> MHHHHHHGSKSVPTAEETRRLAQAM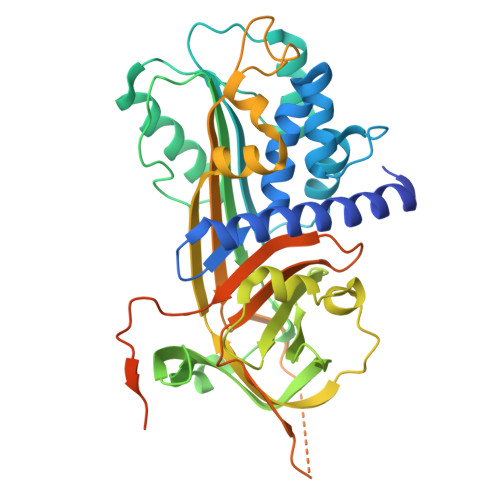MAFTTDLFSLVAQTSTSSNLVLSPLSVALALSHLALGAQNQTLHSLHRVLHMNTGSCLPHLLSHFYQNLGPGTIRLAARIYLQKGFPIKDDFLEQSERLFGAKPVKLTGKQEEDLANINQWVKEATEGKIEDFLSELPDSTVLLLLNAIHFHGFWRTKFDPSLTQKDFFHLDERFTVSVDMMHAVSYPLRWFLLEQPEIQVAHFPFKNNMSFVVVMPTYFEWNVSEVLANLTWDTLYHPSLQERPTKVWLPKLHLQQQLDLVATLSQLGLQELFQGPDLRGISEQNLVVSSVQHQSTMELSEAGVEAAAATSVAMNRMSLSSFTVNRPFLFFIMEDTIGVPLFVGSVRNPNPSALPQLQEQRDSPDNRLIGQNDKADFHGGKTFGPDLKLAPRMEEDYPQFSSPK> GTWIG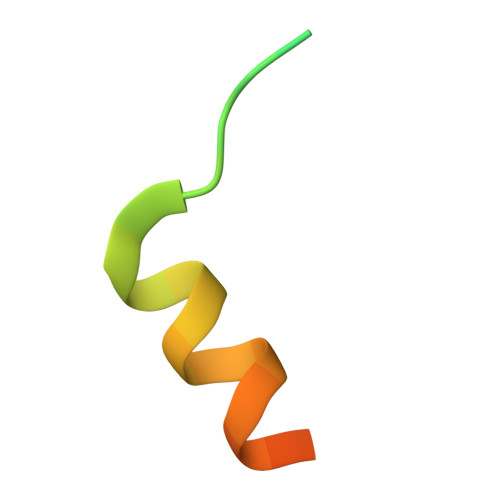EDIFPPLLPPTEQDLTKLLLEGQGESG>[2x]MAVTDLRDVEEDVKGKLDEWLNALVHLDKQQVERIYEELQGEMKHVLDFEIINYYKLLYTRYLIMKRDISALEEELDKLKKVYKKYSPFQKLLYMYGRGLLCCLQYRWKDGLDYLLKTEVMAKEQGYHETGLYYNIALAYTHLDIHHLAIHFVNMALEGFRSEAKARNIINCQILIAVSYTEKGQYEEALKMYESILREATSFADKDVLLAITLSNMGSIYYKKGKYQQAKKYYLDSLQLQKQIDLNYLDTIYEMALVCIKLEELEEARTLIDKGIDAAKQEERFNAKLYLLLMLRYKYFEEAKDYKAFLENEAIPLYKSAGNKIELKKVYVELAEHFSSLSRFEESNRYYRLVIDLMNDNKEERSHHHHHH

Previously, we showed that this process is regulated by the sensor NprR, which, in the presence of its cognate signaling peptide NprX, adopts a tetrameric conformation allowing its binding to specific DNA sequences and transcription of genes involved in survival of the bacteria in insect cadavers. Here, we demonstrate that, in the absence of NprX, NprR is a dimer, which negatively controls sporulation, independently of its transcription factor activity. We show that NprR prevents the phosphorylation of the phosphoprotein Spo0F and inhibits the phosphorylation cascade regulating sporulation. This demonstrates that NprX binding switches the bifunctional sensor NprR from a dimeric sporulation inhibitor to a tetrameric transcription factor. Interestingly, NprR contains both the HTH DNA-binding domain and the two Rap-like additional TPR motifs, and was thus proposed as an evolutionary intermediate in the RNPP family.

We thus used the truncated NprR(ΔHTH) form of the protein, deleted of the HTH domains, which are known to be highly flexible in the absence of DNA. Because crystallisation trials are performed at very high protein concentration favouring the tetrameric form of NprR, we also used the (Y223A/F225A) mutant that has been shown to impair tetramer formation. Crystals were finally obtained with the truncated double mutant protein NprR(ΔHTH)(Y223A/F225A). They diffracted up to 3.25Å resolution in space group P 21 21 21 with 2 molecules per asymmetric unit. In both polypeptide chains contained in the asymmetric unit, the 18 α-helices and the connecting loops forming the 9 TPR motifs of NprR are well defined. The two subunits (called apoA and apoB) display the right-handed superhelix conformation characteristic of TPR domains. They are associated into a stable dimer characterized by an overall interface area of 1113Å2 and a solvation free energy gain ΔiG of -18 kcal/mol. In particular, the dimerization interface involving the C-terminal residues N407 and Y410, which was observed in the NprR/NprX complex, is conserved in the apo dimer. Comparison of the two subunits of the apo NprR dimer demonstrated that, due to distinct crystal packing constraints, the pitch of the superhelix formed by the 9 TPR motifs of the protein is larger in apoB than in apoA. This discrepancy, characterized by a Z-score of 7.9 and an rmsd distance of 1.99Å over 293 aligned Cα atoms, reflects the elasticity of the superhelix and suggests that, in solution and in the absence of NprX, the protein dynamically oscillates between distinct conformations.> IVGGYTCQENSVPYQVSLNSGYHFCGGSLINDQWVVSAAHCYKSRIQVRLGEHNINVLEGNEQFVNAAKIIKHPNFDRKTLNNDIMLIKLSSPVKLNARVATVALPSSCAPAGTQCLISGWGNTLSSGVNEPDLLQCLDAPLL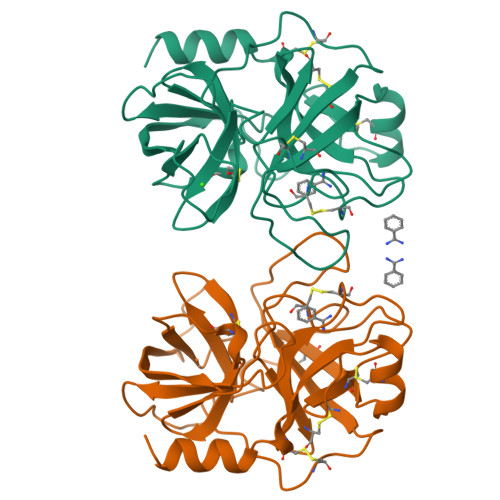PQADCEASYPGKITDNMVCVGFLEGGKDSCQGDSGGPVVCNGELQGIVKWGYGCALPDNPGVYTKVCNYVDWIQDTIAAN The monofunctional counterpart (AAC(6’)-Im) of the acetyltransferase domain of the bifunctional enzyme has been identified in both Gram-negative and Gram-positive clinical isolates 14. It shares 60% sequence identity and 83% similarity with AAC(6’)-Ie. When expressed in the Escherichia coli JM83 strain, AAC(6’)-Im produces resistance to a wide range of clinically important 4,6-disubstituted aminoglycosides with minimal inhibitory concentration (MIC) values 8 - 128-fold above those for the recipient strain. Here we report the antibiotic susceptibility and kinetic profile and the X-ray structure of the AAC(6’)-Im acetyltransferase in its apo form and as the binary kanamycin A complex, and classify the enzyme as a member of the AAC(6’)-I sub-family C. An analysis of the structural features involved in substrate binding provides insight into the modulation of the activity of these enzymes.

The AAC(6’)-Im structure was solved in both the apo-form at 1.7 Å resolution, and as the binary complex with kanamycin A (AAC(6’)-Im-kanamycin A) to 1.95 Å resolution. Superposition of the apo-AAC(6’)-Im and AAC(6’)-Im-kanamycin A structures gives an root-mean-square deviation (rmsd) of 0.6 Å. Inspection of the superimposed structures shows that although there are no major differences in the overall structure of the enzyme upon substrate binding, there are some minor rearrangements of the residues inside the kanamycin binding site. A β-hairpin formed by strand β6’ and the N-terminal end of strand β7 moves inward as a rigid body. In addition, small inward or outward movements of side chains which surround the kanamycin molecule are also observed, primarily to facilitate efficient hydrogen bonding and hydrophobic interactions with the substrate.

>MLEKKRVSFRPMNEDDLVLMLKWLTDDRVLEFYDGRDKKHTQKTIREHYTEQWADEIYRVIIEYDTIPIGYAQIYRIQGELFDEYNYHETEEKIYAMDQFIGEPEYWNMGIGAEYCRVVCQYLRTEMDADAVILDPRKNNLRAVRAYQKAGFKIIKELPEHELHEGKKEDCVLMEWRV[2x]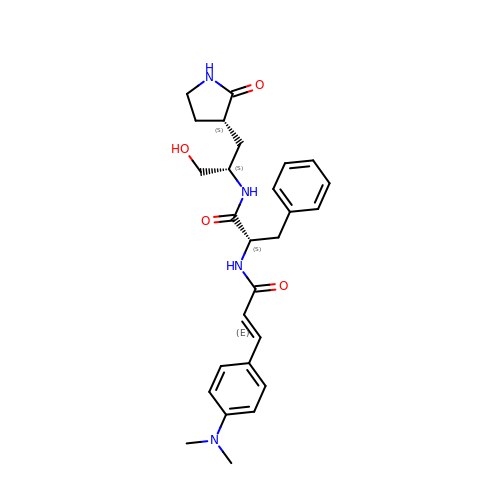(2S)-2-[[(E)-3-[4-(dimethylamino)phenyl]prop-2-enoyl]amino]-N-[(2S)-1-oxidanyl-3-[(3S)-2-oxidanylidenepyrrolidin-3-yl]propan-2-yl]-3-phenyl-propanamide | C27 H34 N4 O4 | MMLGNYLPTJZWEN-XNUWVNOVSA-N Calcium homeostasis modulator 1 (CALHM1) is a voltage-dependent channel involved in neuromodulation and gustatory signaling. CALHM1 is the recently identified member of a large-pore channel that permeates ions, including Ca2+, Na+, K+, and Cl−, and small molecules, such as ATP, in a voltage-dependent manner. Furthermore, the ATP efflux through the CALHM1 channel in type II gustatory cells and the subsequent purinergic signaling has been shown to facilitate the perception of sweet, bitter, and umami taste sensations. Our studies here showed that the human and chicken CALHM1s have a conserved structural fold, oligomeric assembly pattern, and a phospholipid-filled hydrophobic pocket for controlling channel functions.

Second, incorporation of the tryptophan mutation at the ‘entrance’ of the hydrophobic pocket (Ile109Trp) exhibited an approximately five-fold increase in current density compared to the wildtype hCALHM1Δct. To understand the mechanism of functional upregulation in the CALHM1-Ile109Trp mutant (hCALHM1I109W∆ct), we conducted single-particle cryo-EM on this mutant. Our structural analysis revealed that in hCALHM1I109W∆ct, the hydrophobic pocket retains a lipid. Here, the tryptophan residue forms a stronger van der Waals interaction with the lipid than the original isoleucine residue. Indeed, these MD simulations showed that POPC binds more favorably to the hCALHM1I109W∆ct than hCALHM1∆ct (−9.2 kcal/mol in hCALHM1I109W∆ct vs −5.5 kcal/mol in hCALHM1∆ct), supporting the cryo-EM observation that the Ile109Trp mutation stabilizes the POPC binding. The Ile109Trp mutation that upregulates the channel activity binds phospholipids more favorably at the hydrophobic pocket, indicating that the coupling between the phospholipid binding and channel activity. The single-particle cryo-EM on hCALHM1I109W∆ct in the presence of RuR showed oblong density consistent with the size of RuR in the central pore surrounded by the NTHs. Nevertheless, the cryo-EM density is of sufficient quality for the placement of RuR molecule, although an atomic-resolution pose cannot be determined from these data. This density was not observed in the cryo-EM structure of hCALHM1I109W∆ct in the absence of RuR, supporting the view that it represents RuR. Moreover, the structure of hCALHM1I109W∆ct in RuR-free conditions does not clearly resolve the NTHs, indicating a higher degree of conformational flexibility of the NTHs in the absence of RuR. We therefore suggest that the TMD1-Ile109Trp interactions, lipid-Phe19 interactions, and RuR-NTH interactions all contribute towards NTH conformational stabilization.

>[8x]MMDKFRMIFQFLQSNQESFMNGICGIMALASAQMYSAFDFNCPCLPGYNAAYSAGILLAPPLVLFLLGLVMNNNVSMLAEEWKRPPGRRAKDPAVLRYMFCSMAQRALWAPVVWVAVTLLDGKCFLCAFCTAVPVSALGNGSLAPGLPAPELARLLARVPCPEIYDGDWLLAREVAVRYLRCISQALGWSFVLLTTLLAFVVRSVRPCFTQAAFLKSKYWSHYIDIERKLFDETCTEHAKAFAKVCIQQFFEAMNHDLELGHTNGTLATAPASAAAPTTPDGAEEEREKLRGITDQGTMNRLLGSAWSHPQFEK>[2x]NNNGA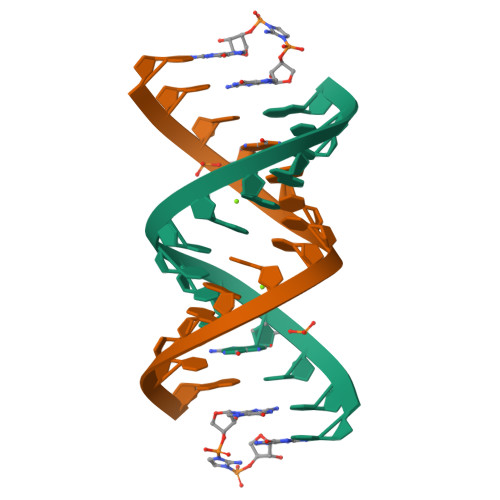CUUAAGUCG> R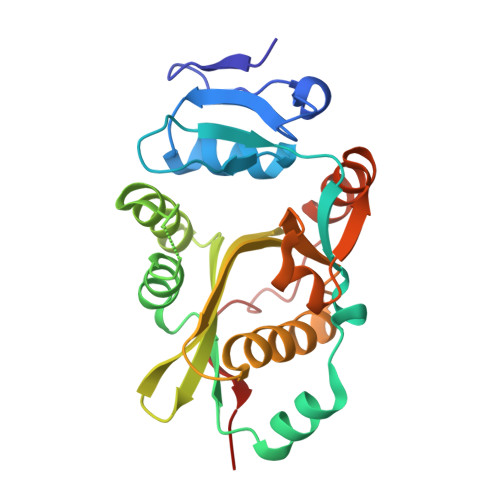LVQLSRHSIAFPSPEGALREPNGLLALGGDLSPARLLMAYQRGIFPWFSPGDPILWWSPDPRAVLWPESLHISRSMKRFHKRSPYRVTMNYAFGQVIEGCASDREEGTWITRGVVEAYHRLHELGHAHSIEVWREDELVGGMYGVAQGTLFCGESMFSRMENASKTALLVFCEEFIGHGGKLIDCQVLNDHTASLGACEIPRRDYLNYLNQMRLGRLPNNFWVPRCLFSPQE(2~{R})-2-methyl-2-methylsulfonyl-4-[6-[2-[4-(morpholin-4-ylmethyl)phenyl]ethynyl]-3-oxidanylidene-1~{H}-pyrrolo[1,2-c]imidazol-2-yl]-~{N}-oxidanyl-butanamide | C25 H30 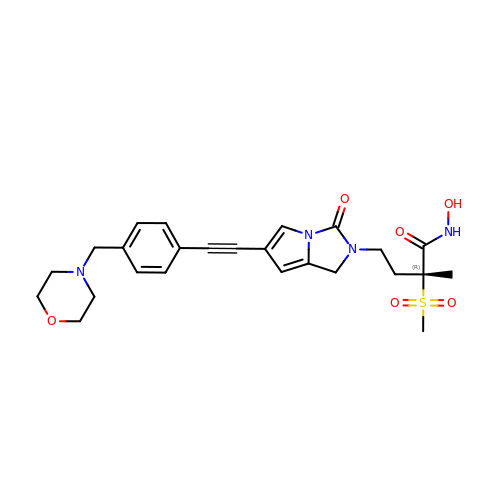N4 O6 S | HKFPYIZPYVWIPB-RUZDIDTESA-N>MATTTVGLTDLKVRLVRDDFADAVAWVARSLPSRPTVPVLAGVLLTGSDDGLTISSFDYEVSAEVQIPAEIAAPGTVLVSGRLLSEITRALPNKPVDLSVEGTRVSLTCGSARFSLPTMAVEDYPALPELPAETGSVPADLFAEAIGQVAVAAGRDDTLPMLTGIRVEISGDRMVLAATDRFRLAVRELTWTTKTPDVEAAVLVPAKTLAEAAKTGLDGSEVQLALGAGPSVGQDGLLGIRSEGKRSTTRLLDAEFPKFRQLLPTEHTAMATIGVGELTEAIKRVALVADRGAQVRMEFADDVLHLSAGADDVGRAEEDLPVSFSGEPLTIAFNP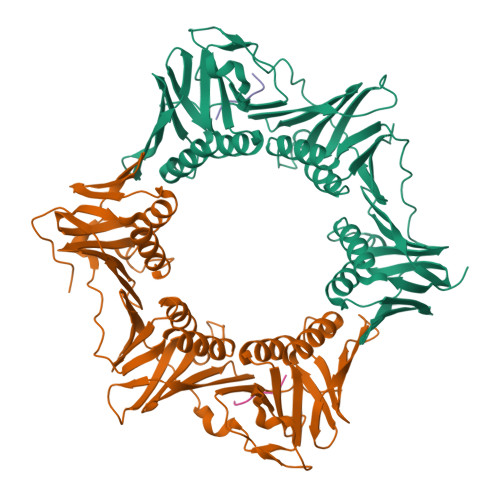GYLTDGLGALHSERVTFGFTTPSKPAVLRPATEADAALNGNGPFPAAETDYVYLLMPVRLPG[4x];>QFDLFG[4x]> ENNCLNAAKACNLNDTCKKYRSAYISPCTSRVST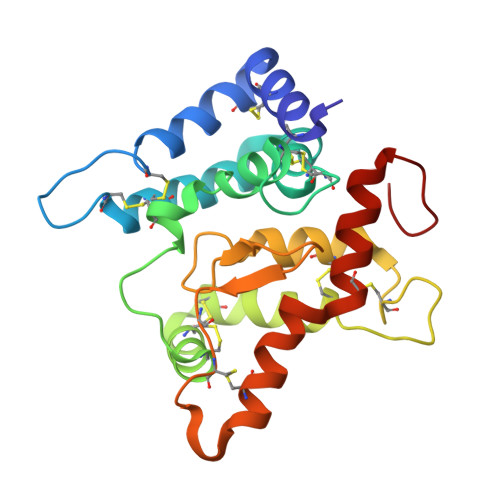AEVCNKRKCHKALRQFFDKVPPKHSYGMLYCSCPLGDQSACSERRRQTIVPACSYEDKERPNCLTLQVSCKTNYICRSRLADFFTNCQPEPLSLSGCLKENYADCLLSYSGLIGTVMTPNYLRSPKISVSPFCDCSSSGNSKEECDRFTEFFTDNACLRNAIQAFGNGTGSEFLE(3R)-3-hydroxy-2,4-dioxopentyl dihydrogen phosphate | C5 H9 O7 P | 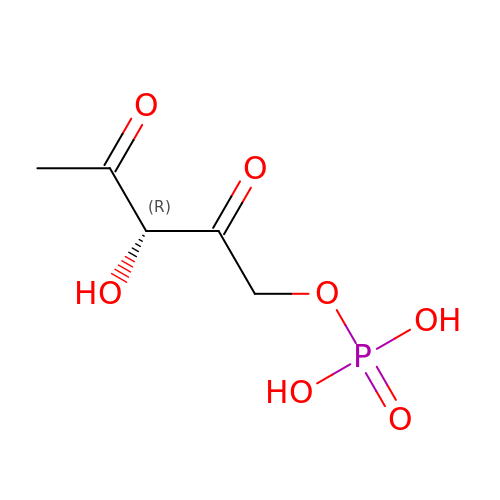AKHNGSPNHAFBII-RXMQYKEDSA-N>[2x]MEEPEEPADSGQSLVPVYIYSPEYVSMCDSLAKIPKRASMVHSLIEAYALHKQMRIVKPKVA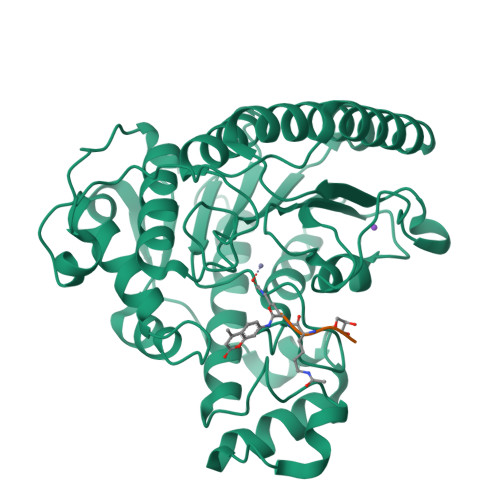SMEEMATFHTDAYLQHLQKVSQEGDDDHPDSIEYGLGYDCPATEGIFDYAAAIGGATITAAQCLIDGMCKVAINWSGGWHHAKKDEASGFCYLNDAVLGILRLRRKFERILYVALDLHHGDGVEDAFSFTSKVMTVSLHKFSPGFFPGTGDVSDVGLGKGRYYSVNVPIQDGIQDEKYYQICESVLKEVYQAFNPKAVVLQLGADTIAGDPMCSFNMTPVGIGKCLKYILQWQLATLILGGGGFNLANTARCWTYLTGVILGKTLSSEIPDHEFFTAYGPDYVLEITPSCRPDRNEPHRIQQILNYIKGNLKHVVIEGRGSHHHHHH>GSSHSSANEDMPVERILEAELAVEPKTETYVEANMGLNPSSPNDPVTNICQAADKQLFTLVEWAKRIPHFSELPLDDQVILLRAGWNELLIASFSHRSIAVKDGILLATGLHVHRNSAHSAGVGAIFDRVLTELVSKMRDMQMDKTELGCLRAIVLFNPDS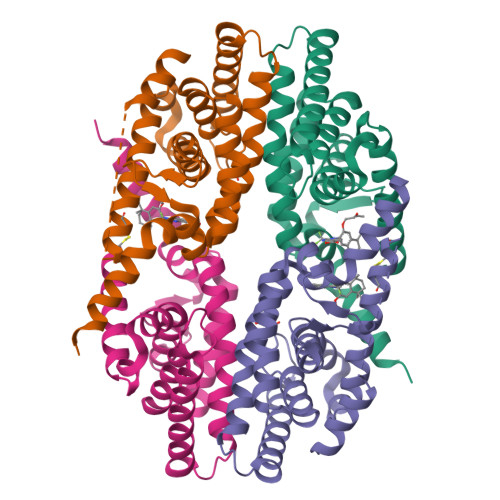KGLSNPAEVEALREKVYASLEAYCKHKYPEQPGRFAKLLLRLPALRSIGLKCLEHLFFFKLIGDTPIDTFLMEMLEAPHQMT[4x]>GAMDPMICLGLEGTAEKTGVGIVTSDGEVLFNKTIMYKPPKQGINPREAADHHAETFPKLIKEAFEVVDKNEIDLIAFSQGPGLGPSLRVTATVARTLSLTLKKPIIGVNHCIAHIEIGKLTTEAEDPLTLYVSGGNTQVIAYVSKKYRVFGETLDIAVGNCLDQFARYVNLPHPGGPYIEELARKGKKLVDL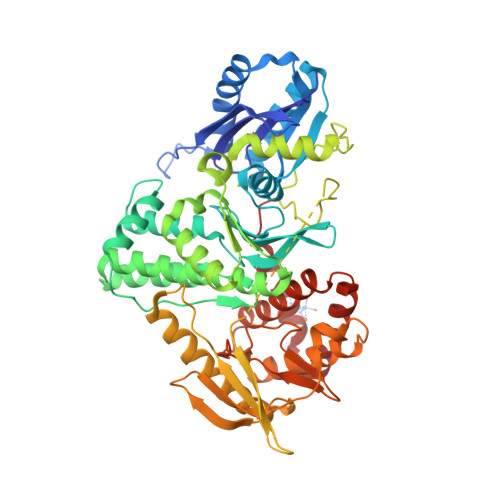PYTVKGMDIAFSGLLTAAMRAYDAGERLEDICYSLQEYAFSMLTEITERALAHTNKGEVMLVGGVAANNRLREMLKAMCEGQNVDFYVPPKEFCGDNGAMIAWLGLLMHKNGRWMSLDETKIIPNYRTDMVEVNWIKEIKGKKRKIPEHLIGKGAEADIKRDSYLDFDVIIKERVKKGYRDERLDENIRKSRTAREARYLALVKDFGIPAPYIFDVDLDNKRIMMSYINGKLAKDVIEDNLDIAYKIGEIVGKLHKNDVIHNDLTTSNFIFDKDLYIIDFGLGKISNLDEDKAVDLIVFKKAVLSTHHEKFDEIWERFLEGYKSVYDRWEIILELMKDVERRARYVE[2x]>[2x]SNAMKKFSVVIAGGGSTFTPGIVLMLLANQDRFPLRSLKFYDNDGARQETIAEACKVILKEQAPEIEFSYTTDPQAAFTDVDFVMAHIRVGKYPMREQDEKIPLRHGVLGQETCGPGGIAYGMRSIGGVLELVDYMEKYSPNAWMLNYSNPAAIVAEATRRLRPNAKILNICDMPIGIEGRMAQIVGLKDRKQMRVRYYGLNHFGWWTSIEDLDGNDLMPKLREYVAKYGYVPPSNDPHTEASWNDTFAKAKDVQALDPQTMPNTYLKYYLFPDYVVAHSNPERTRANEVMDHREKNVFSACRAIIAAGKSTAGDLEIDEHASYIVDLATAIAFNTQERMLLIVPNNGAIHNFDADAMVEIPCLVGHNGPEPLTVGDIPHFQKGLMSQQVAVEKLVVDAWEQRSYHKLWQAITLSKTVPSASVAKAILDDLIAANKDYWPELH

Here, we report the deposition of 14 structures of enzymes from both the core and accessory genomes of sequence type 23 (ST23) K1 hypervirulent K. pneumoniae. Targets were selected using a shotgun approach aimed at uncharacterized metabolic proteins from ST23 K1 hypervirulent K. pneumoniae. In silico multilocus sequence typing of all K. pneumoniae isolates was completed using Kleborate. This analysis showed that 64 of the selected proteins are part of the K. pneumoniae core genome, defined as genes present in at least 95% of all strains; the other 132 proteins are part of the K. pneumoniae accessory genome and are overrepresented in the highly virulent hvKp clonal group CG23, which contains ST23 (7). Thus, the x-ray crystal structures presented here provide the basis for functional analysis of 12 uncharacterized proteins associated with high-risk K. pneumoniae infection.

Of these targets, 34 were successfully purified from large-scale preparations and entered crystallization trials. Fourteen structures were determined for 13 different targets as detailed in Fig. 1.> GAMGSGNQTRALLDDQARHLLTEQERATMMYYLAQYRGGTISVEAMVMALFELLNTHA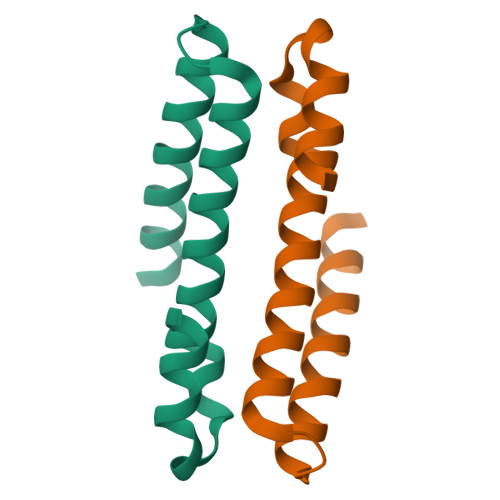KFSLLSEVRSIISPQDLDRFDHLVLRR>[2x]MQAQLQRPRTTGMLVIMASLMVGTPMAMAAKSSSLDAPQQLQVPTLAYDESSIVLVWKAPEDTRKIVDYQIFSAGKLLGKASDNNDNFSPAKPYIDHFYVNDKDNFQHKIVMQNFTVIGLKPETSYQFTVKAQYADGSLSVASKPITAKTSAKPQIVNVRDFGAIDDGKTLNTKAIQQAIDSCKPGCRVEIPAGTYKSGALWLKSDMTLNLQAGAILLGSENPDDYPAG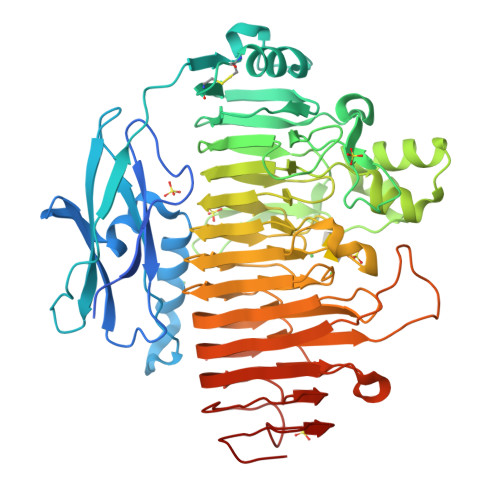YRLYPYSTIERPASLINAIDPNNSKPGTFRNIRITGSGVIDGNGWLRAKTAEITDELGRSLPQYVASKNSKVHEDGILAKNQVEKAVSDGMDLKNAYGQRRSSLMTLRGVENVYLAGFTVRNPAFHGIMNLENHNVVANGLIHQTYDANNGDGIEFGNSQNVMVFNNFFDTGDDCINFAAGTGEKAQEQEPMKGAWLFNNYFRMGHGAIVTGSHTGAWIEDILAENNVMYLTDIGLRAKSTSTIGGGARNVTFRNNAMRDLAKQVMVMTLDYADSNANIDYPPAKIPAQFYDFTLKNVTVDNSTGKNPSIEIKGDTANKAWHRLVHVNNVQLNNVTPTAISDLRDSEFNKVTFTELRGDTPWHFSEVKNVKVDGKPVAP> ETITVSTPIKQIFPDDAFAETIKDNLKKKSVTDAVTQNELNSIDQIIANNSDIKSVQGIQYLPNVTKLFLNGNKLTDIKPLTNLKNLGWLFLDENKIKDLSSLKDLKKLKSLSLEHNGISDINGLVHLPQLESLYLGNNKITDITVLSRLTKLDTLSLE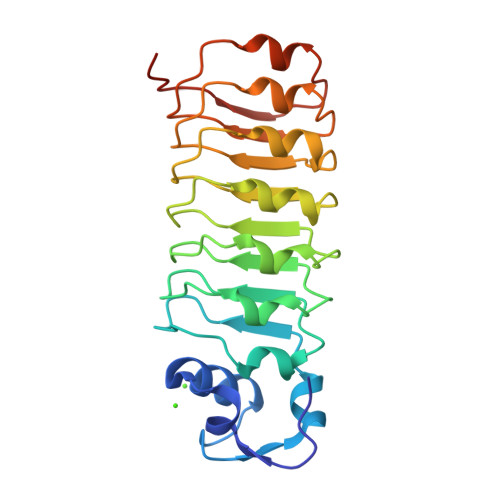DNQISDIVPLAGLTKLQNLYLSKNHISDLRALAGLKNLDVLELFSQECLNKPIN The Marasmius oreades agglutinin (MOA) is the holotype of an emerging family of fungal chimerolectins and an active Ca2+/Mn2+-dependent protease, which exhibits a unique papain-like fold with special active site features. While acting as a dimerization domain, the papain-like domain of MOA retains the characteristic L-/R-domain partition of PLCPs. As additional feature, the MOA dimer carries two binuclear metal-binding clusters, symmetrically placed at the dimerization interface (Grahn et al., 2009). MOA requires the presence of calcium or manganese (II) to switch from the inactive form to an active protease (Cordara et al., 2011, Wohlschlager et al., 2011).

In an effort to validate our substrate binding model, we co-crystallized the enzymatically inactive MOA variants C215A and C215A/H257A with two synthetic heptapeptides mimicking proteolytic substrates. The designed peptides have the sequence PVxRAHS (with x = P or V). To our surprise, the co-crystallized peptide probes were cleaved in both structures, despite the fact that we used catalytically inactive enzymes. The observed cleavage products correspond to the N-terminal proteolytic fragments, binding to the MOA active site in the standard backbone orientation expected for PLCP substrates. Throughout subsites S1–S4, the peptides match the proposed MOA substrate model derived from the MOA-bound Z-VAD-fmk inhibitor complex (Cordara et al., 2016). The synthetic peptides are anchored to the active site through three main contact points: the oxyanion hole, defined by Trp208 and the backbone NH group of Ala215, the ‘site B’ Ca2+ ion and a backbone–backbone interaction with Ala256. The presence of an arginine residue at the P1 position unambiguously maps the S1 subsite to the carboxylate group of L-domain Glu210, which forms a side-on bidentate salt bridge with the Arg guanidinium group. The P2 moiety binds to the S2 specificity pocket lined by residues Leu247, Ala258 and Leu182# (with ‘#’ identifying a residue provided by the other subunit). Coupled to the long time needed to grow the crystals (2–3 weeks), this could explain the presence of a cleaved peptide rather than the full substrate. The peptide fragment occupies the S1–S4 subsites of the catalytic cleft and matches the N-terminal part of the expected proteolytic product, representing a snapshot of MOA just after the acylation step, mediated by a water molecule in the absence of the Cys nucleophile (Fig. 6 frame 3). A stretch of poorly defined electron density close to subsites S1′-S3′ suggests the lingering presence of the C-terminal fragment of the cleaved substrate.

> MSLRRGIYHIENAGVPSAIDLKDGSSSDGTPIVGWQFTPDTINWHQLWLAEPIPNVADTFTLCNLFSGTYMDLYNGSSEAGTAVNGWQGTAFTTNPHQLWTIKKSSDGTSYKIQNYGSKTFVDLVNGDSSDGAKIAGWTGTWDEGNPHQKWYFNRMSVSSAEAQAAIARNPHIHGTYRGYILDGEYLVLPNATFTQIWKDSGLPGSKWREQIYDADDFAIAMKAAVGKWGADSWKANGFAIFCGVMLGVNKAGDAAHAYNFTLTKDHADIVFFEPQNGGYLNDIGYDSYMAFY;> PVPR> GSHMEVLKNIRIYPLSNFITSTKNYINLPNELRNLISEEQESKLGFLHIIESDFKPSVALQKLVNCTTGDEKILIIDIVSIWSQQKQRQHGAIYMNSLSCINITGLIVFLELLYDSPMDALRRCQVDNFNFQLRGIVIDNLSFLNFESDKNYDVINLSKFEKLFKILRKLREFLGCWIITKSFPTDFYNGIENTLVDKWSIKRKSGVTLYPTKLPDSYMKGMDLIIYREVVDGRPQYRRIAALEE;> MEYEDLELITIWPSPTKNKLCQFIKQNLSKEHVVTQLFFIDATSSFPLSQFQKLVPPTLPENVRIYENIRINTCLDL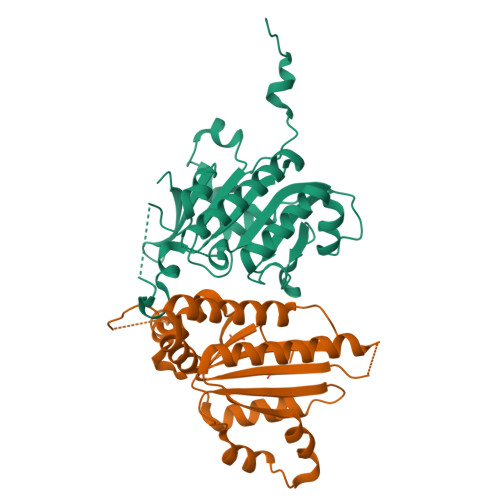EELSAITVKLLQILSMNKINAQRGTEDAVTEPLKIILYINGLEVMFRNSQFKSSPQRSHELLRDTLLKLRVMGNDENENASIRTLLEFPKEQLLDYYLKKNNNTRTSSVRSKRRRIKNGDSLAEYIWKYYADSLFE>[2x]MDFLRNLFSQTLSLGSQKERLLDELTLEGVARYMQSERCRRVICLVGAGISTSAGIPDFRSPSTGLYDNLEKYHLPYPEAIFEISYFKKHPEPFFALAKELYPGQFKPTICHYFMRLLKDKGLLLRCYTQNIDTLERIAGLEQEDLVEAHGTFYTSHCVSASCRHEYPLSWMKEKIFSEVTPKCEDCQSLVKPDIVFFGESLPARFFSCMQSDFLKVDLLLVMGTSLQVQPFASLISKAPLSTPRLLINKEKAGQSDPFLGMIMGLGGGMDFDSKKAYRDVAWLGECDQGCLALAELLGWKKELEDLVRREHASIDAQS;>[2x]PKKTG

Sirtuins, which are represented by the founding member yeast SIR2 (silencing information regulator 2), are a class of enzymes that possess Nicotinamide Adenine Dinucleotide (NAD+)-dependent protein lysine deacetylase activity and were originally discovered in the aging and epigenetic fields. Mammals possess seven sirtuins, SIRT1-75, which share a conserved catalytic core domain but differ in their N- and C- termini. SIRT2 is the only primarily cytoplasmic isoform6; however, it has also been observed in the nucleus. Our study reveals that SIRT2 prefers myristoyl lysine as a substrate slightly over acetyl lysine.

Upon screening of crystallization conditions, we obtained crystals of SIRT2 in complex with a thiomyristoyl peptide, referred to as BHJH-TM1. BHJH-TM1 was synthesized as a mechanism-based inhibitor of SIRT1-3 and SIRT616. The crystal structure of SIRT2/BHJH-TM1 was refined to a resolution of 2.1 Å, with two subunits in the asymmetric unit. As observed in the crystal structures of apo SIRT2 and other sirtuins, SIRT2/BHJH-TM1 consists of two distinct domains: a Rossmann fold domain and a zinc-binding domain. The BHJH-TM1 peptide (PKK(TMy)TG) consists of five amino acid residues with a thiomyristoyl group attached to the central lysine residue. The BHJH-TM1 peptide fits well into a long stretch of electron density observed between the N-terminal Rossmann fold domain and C-terminal zinc-binding domain of SIRT2. The thiomyristoyl group of BHJH-TM1 is accommodated by a hydrophobic pocket formed by several hydrophobic residues of SIRT2, including Ile93, Phe96, Phe119, Phe131, Leu134, Leu138, Phe143, Ile169, Phe190, Ile232, and Phe234. The extensive hydrophobic interactions between the thiomyristoyl group and SIRT2 may account for the much lower Km value of SIRT2 toward the myristoyl lysine peptide. Comparison of the active sites of SIRT2/BHJH-TM1 and apo SIRT2 reveals that the hydrophobic residues from the Rossmann fold domain that form the myristoyl pocket (e.g., Ile93, Phe143, and Ile169) superpose relatively well, whereas the hydrophobic residues from the zinc-binding domain (e.g., Phe131, Leu138, and Phe234) move approximately 3–4 Å between the apo SIRT2 structure and the SIRT2/BHJH-TM1 structure. This conformational change reshapes the binding site, which may better accommodate the thiomyristoyl group.>[2x]QDTFIAAVYEHAAILPNATLTPVSREEALALMNRNLDILEGAITSAADQGAHIIVTPEDAIYGWNFNRDSLYPYLEDIPDPEVNWIPCNNRNRFGQTPVQERLSCLAKNNSIYVVANIGDKKPCDT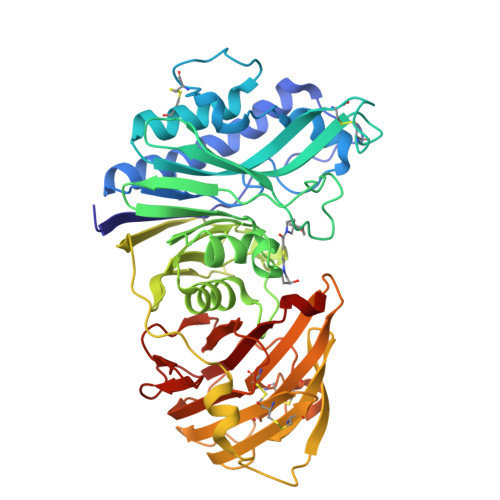SDPQCPPDGRYQYNTDVVFDSQGKLVARYHKQNLFMGENQFNVPKEPEIVTFNTTFGSFGIFTCFDILFHDPAVTLVKDFHVDTIVFPTAWMNVLPHLSAVEFHSAWAMGMRVNFLASNIHYPSKKMTGSGIYAPNSSRAFHYDMKTEEGKLLLSQLDSHPSHSAVVNWTSYASSIEALSSGNKEFKGTVFFDEFTFVKLTGVAGNYTVCQKDLCCHLSYKMSENIPNEVYALGAFDGLHTVEGRYYLQICTLLKCKTTNLNTCGDSAETASTRFEMFSLSGTFGTQYVFPEVLLSENQLAPGEFQVSTDGRLFSLKPTSGPVLTVTLFGRLYEKD>HMTDGERQNATEIRASVGKMIDGIGRFYIQMCTELKLSDYEGRLIQNSLTIERMVLSAFDERRNKYLEEHPSAGKDPKKTGGPIYRRVDGKWRRELILYDKEEIRRIWRQANNGDDATAGLTHMMIWHSNLNDATYQRTRALVRTGMDPRMCSLMQGSTLPRRSGAAGAAVKGVGTMVMELIRMIKRGINDRNFWRGENGRRTRIAYERMCNILKGKFQTAAQRTMVDQVRESRNPGNAEFEDLIFLARSALILRGSVAHKSCLPACVYGSAVASGYD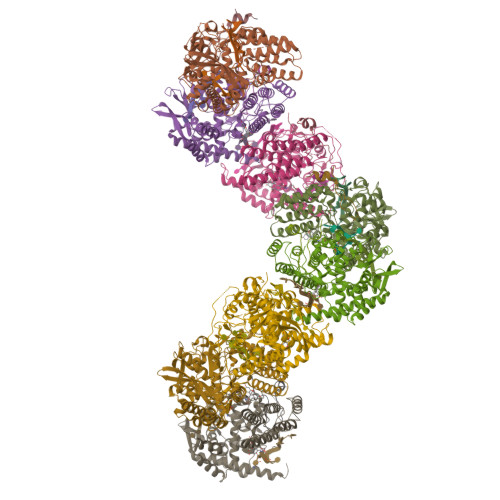FEREGYSLVGIDPFRLLQNSQVYSLIRPNENPAHKSQLVWMACHSAAFEDLRVSSFIRGTKVVPRGKLSTRGVQIASNENMETMESSTLELRSRYWAIRTRSGGNTNQQRASSGQISIQPTFSVQRNLPFDRPTIMAAFTGNTEGRTSDMRTEIIRLMESARPEDVSFQGRGVFELSDEKATSPIVPSFDMSNEGSYFFGDNAEEYDNLEHHHHHH[2x]> GLPTMNTPGSCQFLTSDDFQSPSAMPQYDVTPEMRIPGEVKNLMEIAEVDSVVPVQNVGEKV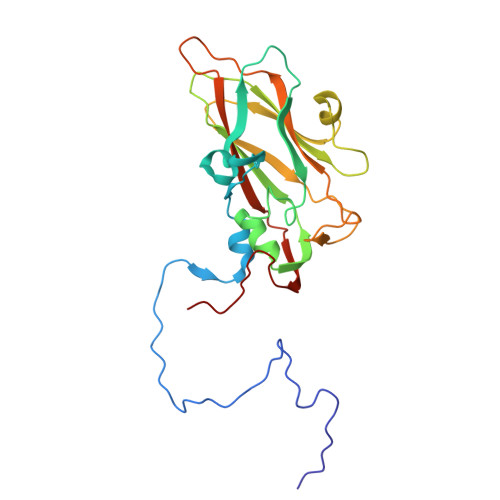NSMEAYQIPVRSNEGSGTQVFGFPLQPGYSSVFSRTLLGEILNYYTHWSGSIKLTFMFCGSAMATGKFLLAYSPPGAGAPTKRVDAMLGTHVVWDVGLQSSCVLCIPWISQTHYRYVASDEYTAGGFITCWYQTNIVVPADAQSSCYIMCFVSACNDFSVRLLKDTPFITQQNFFQ> TRDQNGTWEMESNENFEGYMKALDIDFATRKIAVRLTQTLVIDQDGDNFKFKTTSTFRNYDVDFTVGVEFDEYTKSLDNRHVKALVTWEGDVLVCVQKGEKENRGWKKWIEGDKLY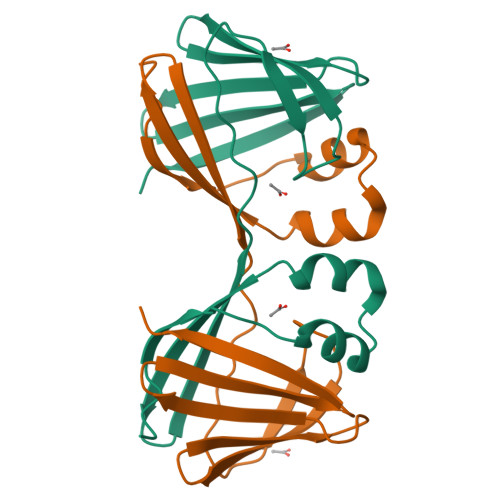LELTCGDQVCRQVFKKK~{N}-cyclohexyl-4-methyl-piperidine-1-carboxamide | C13 H24 N2 O | 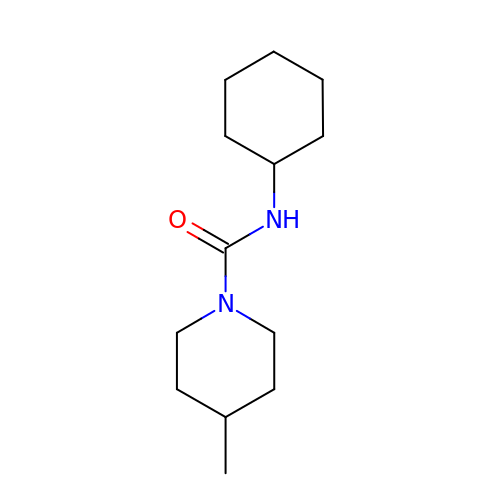BOSHLBWKQSSSGD-UHFFFAOYSA-N Shiga toxin (Stx), a major virulence factor of enterohemorrhagic Escherichia coli (EHEC), can cause fatal systemic complications. All Stx proteins consist of a catalytic A-subunit and a B-subunit pentamer. The catalytic A-subunit, which is a member of ribosome-inactivating proteins (RIPs), has an RNA N-glycosidase activity that cleaves a specific adenine from 28S ribosomal RNA to inhibit eukaryotic protein synthesis. The B-subunit pentamer functions to bind Galα[1–4]–Galβ[1–4]–Glcβ-ceramide (Gb3), a glycolipid present on the surface of target cells.

To elucidate the precise manner by which these shorter peptides bind to Stx2a, X-ray crystallography analysis was performed with co-crystals of each peptide and the Stx2a holotoxin, which were obtained via the soaking method. We were able to determine electron densities for AR4A-mono, R4A-mono, R3A-mono, and R2A-mono, and X-ray crystal structures were solved to final resolutions of 1.80, 1.80, 1.90, and 1.75 Å-resolution, respectively. These structures reveal that the AR4A-mono, R4A-mono, R3A-mono, and R2A-mono peptides bind tightly to the catalytic A-subunit. In all cases, the common Arg8-Arg9-Ala10 motif (numbering reflects residue position in full-length MMβA-mono) interacts equally with the Glu72, Tyr77, Val78, Asp94, Ser112, Tyr114, Thr115, Glu167, Arg170, Thr199, and Gly203 residues present in the catalytic pocket of the A-subunit, whereas the Arg8 and Arg9 residues of the motif electrostatically interact with Glu167 and Asp94, respectively. The amide group of the Ala10, but not its side chain, interacts with the Val78, Ser112 and Arg170 residues. In addition, Arg6 and Arg7 of both AR4A-mono and R4A-mono electrostatically interact, respectively, with Asp94 of the A-subunit and Asp70 of the B-subunit, which is adjacent to the catalytic cavity. Overall, we find that the binding patterns of these shorter peptides are almost identical to that of MMβA-mono. We found that R4-mono, AR4A-mono, R4A-mono, and R3-mono exhibit greater inhibitory effects (relative IC50 values = 0.387, 2.27, 2.70, and 3.68 µM, respectively) than non-tagged MMβA-mono (relative IC50 = 8.14 µM), which was used as a positive control to compete the binding. Although the precise mechanism of the detrimental effect of the C-terminal Ala is remained to be elucidated, the presence of the amide group of the C-terminal Ala may contribute to fix the binding manner of the peptides with this Ala, such as MMbA-mono, AR4A-mono, R4A-mono, R3A-mono, and R2A-mono, to the same orientations which are clearly demonstrated in their crystal structures.

> REFTIDFSTQQSYVSSLNSIRTEISTPLEHISQGTTSVSVINHTPPGSYFAVDIRGLDVYQARFDHLRLIIEQNNLYVAGFVNTATNTFYRFSDFTHISVPGVTTVSMTTDSSYTTLQRVAALERSGMQISRHSLVSSYLALMEFSGNTMTRDASRAVLRFVTVTAEALRFRQIQREFRQALSETAPVYTMTPGDVDLTLNWGRISNVLPEYRGEDGVRVGRISFNNISAILGTVAVILNCHHQGARSVRAVNEESQPECQITGDRPVIKINNTLWESNTAAAFLNRKSQFLYTTGK;>[5x]ADCAKGKIEFSKYNEDDTFTVKVDGKEYWTSRWNLQPLLQSAQLTGMTVTIKSSTCESGSGFAEVQFNND;> RRRRAX(2E)-2-[({3-hydroxy-2-methyl-5-[(phosphonooxy)methyl]pyridin-4-yl}methyl)imino]-4-(methylsulfanyl)butanoic 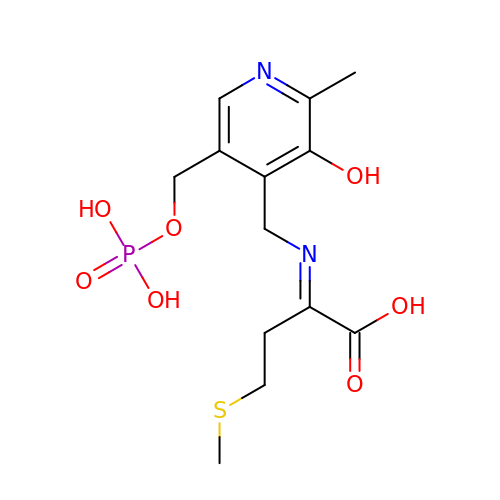acid | C13 H19 N2 O7 P S | RNHGWTJOZCEIDD-RVDMUPIBSA-N> MHHHHHHSSGRENLYFQGGVIESNWNEIVDNFDDMNLKESLLRGIYAYGFEKPSAIQQRAIIPCIKGYDVIAQAQSGTGKTATFAISILQQLEIEFKETQALVLAPTRELA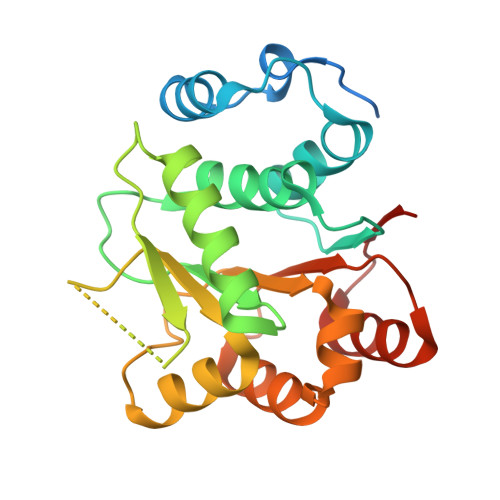QQIQKVILALGDYMGATCHACIGGTNVRNEMQKLQAEAPHIVVGTPGRVFDMLNRRYLSPKWIKMFVLDEADEMLSRGFKDQIYEIFQKLNTSIQVVLLSATMPTDVLEVTKKFMRDPIRILVKKE> MWFLYGCCLRFVLFVLCYYMSPRLPSSGNRRVLYAVFYLYIFVWCVRCFFCGIFILSFALFI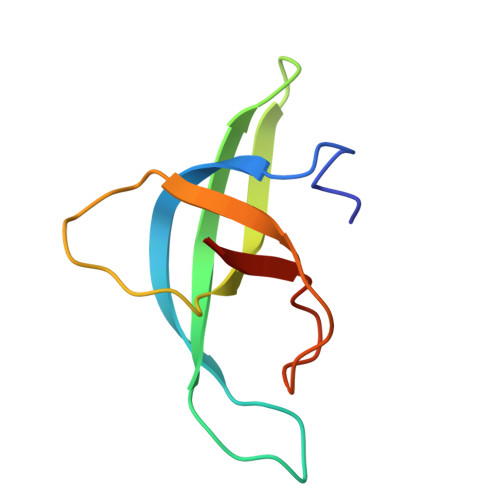IEGGGFIDLPGIKYYTRICY>MEFGFFDDANKEYVITVPRTPYPWINYLGTENFFSLISNTAGGYCFYRDARLRRITRYRYNNVPIDMGGRYFYIYDNGDFWSPGWSPVKRELESYECRHG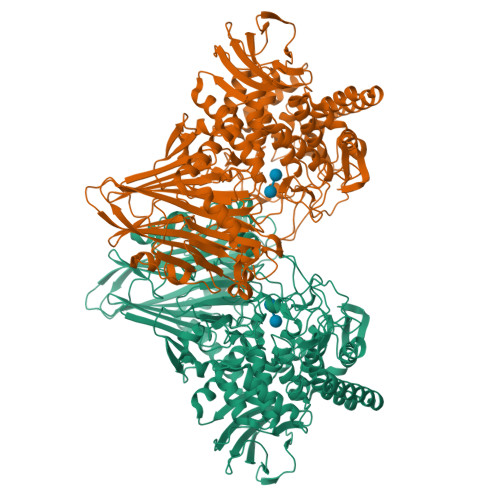LGYTKIAGKRNGIKAEVTFFVPLNYNGEVQKLILKNEGQDKKKITLFSFIEFCLWNAYDDMTNFQRNFSTGEVEIEGSVIYHKTEYRERRNHYAFYSVNAKISGFDSDRDSFIGLYNGFDAPQAVVNGKSNNSVADGWAPIASHSIEIELNPGEQKEYVFIIGYVENKDEEKWESKGVINKKKAYEMIEQFNTVEKVDKAFEELKSYWNALLSKYFLESHDEKLNRMVNIWNQYQCMVTFNMSRSASYFESGIGRGMGFRDSNQDLLGFVHQIPERARERLLDLAATQLEDGSAYHQYQPLTKKGNNEIGSNFNDDPLWLILATAAYIKETGDYSILKEQVPFNNDPSKADTMFEHLTRSFYHVVNNLGPHGLPLIGRADWNDCLNLNCFSTVPDESFQTTTSKDGKVAESVMIAGMFVFIGKDYVKLCEYMGLEEEARKAQQHIDAMKEAILKYGYDGEWFLRAYDDFGRKVGSKENEEGKIFIESQGFCVMAEIGLEDGKALKALDSVKKYLDTPYGLVLQNPAFTRYYIEYGEISTYPPGYKENAGIFCHNNAWIICAETVVGRGDMAFDYYRKIAPAYIEDVSDIHKLEPYVYAQMVAGKDAKRHGEAKNSWLTGTAAWNFVAISQWILGVKPDYDGLKIDPCIPKAWDGYKVTRYFRGSTYEITVKNPNHVSKGVAKITVDGNEISGNILPVFNDGKTHKVEVILEHHHHHH[2x]> MHKFTGVNAKFQQPALRNLSPVVVEREREEFVGFFPQ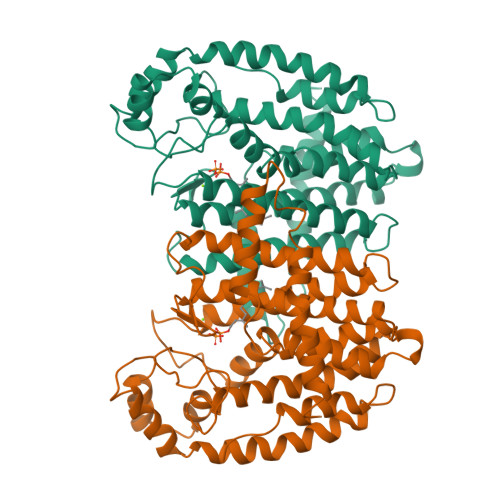IVRDLTEDGIGHPEVGDAVARLKEVLQYNAPGGKCNRGLTVVAAYRELSGPGQKDAESLRCALAVGWCIELFQAASLVADDIMDQSLTRRGQLCWYKKEGVGLDAINDSFLLESSVYRVLKKYCRQRPYYVHLLELFLQTAYQTELGQMLDLITAPVSKVDLSHFSEERYKAIVKYKTAFYSFYLPVAAAMYMVGIDSKEEHENAKAILLEMGEYFQIQDDYLDCFGDPALTGKVGTDIQDNKCSWLVVQCLQRVTPEQRQLLEDNYGRKEPEKVAKVKELYEAVGMRAAFQQYEESSYRRLQELIEKHSNRLPKEIFLGLAQKIYKRQK> NGGVGVDVELITSINVENDTFIERNFTPQEIEYCSAQPSVQSSFAGTWSAKEA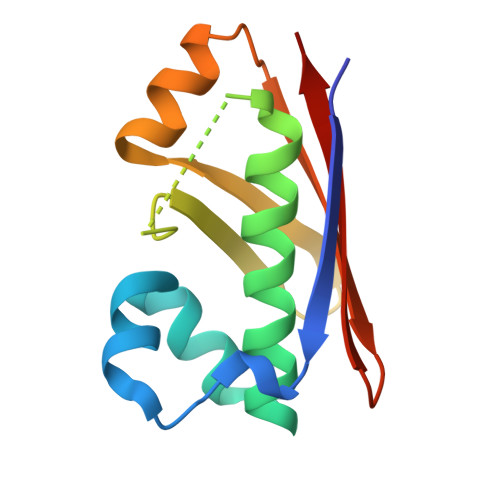VFKSLGVKSLGGGAALKDIEIVRVNKNAPAVELHGNAKKAAEEAGVTDVKVSISHDDLQAVAVAVSTKK3-[2-fluoro-5-(trifluoromethyl)phenyl]-7-methyl-1-[(2-methyl-2H-tetrazol-5-yl)methyl]-1H-indazole | C18 H14 F4 N6 | 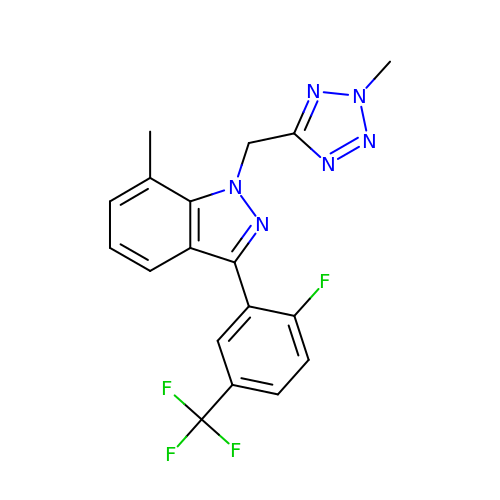MMEFXWUINPSTPN-UHFFFAOYSA-N The first gene encodes the nucleoprotein (N protein) which associates with the viral genomic and antigenomic RNAs to form the helical nucleocapsid. The paramyxoviral nucleocapsid assembly entirely covers the viral genome, protecting it from detection and degradation by host factors and serving as the template for viral mRNA transcription and genome replication. Here, we determined the cryoEM structure of the recombinantly expressed, full-length, and tag-free HeV N protein in complex with E. coli host-derived RNA. Following cryoEM data collection, a multimeric HeV N protein double-ring assembly was resolved to 3.5 Å resolution, enabling the building and refinement of an atomic HeV N protein model.

Subsequent 3D refinement of a curated particle stack comprising 5638 particles and using D14 symmetry resulted in a 3.5 Å resolution cryoEM density map, revealing a previously uncharacterised multimeric nucleoprotein assembly. In the HeV N protein assembly two rings stack ‘bottom-to-bottom’, where the globular N-terminal domains (NTDs) intercalate to form a dimer of tetradecamers. Each tetradecameric ring has a diameter of approximately 20 nm and is topped with the C-terminal arms (Ct-arms) which cover parts of the globular C terminal domains (CTDs). The double ring assembly is approximately 12.5 nm tall, and each ring has an aperture formed by the Ct-arms that is approximately 7 nm wide. The HeV N protein double-ring assembly is formed through extensive lateral interactions in each tetradecameric ring as well as intercalating interactions between two tetradecameric rings. A defining feature of this HeV N protein double-ring assembly is the gear-wheel interface between the two tetradecameric rings. This intercalation zone consists solely of residues in the NTDs of N protomers in the top ring and N protomers in the bottom ring (indicated by the lower-case n). The Ni protomer contacts two protomers in the bottom ring (ni and ni+1), with a total calculated buried surface area of ~ 545 Å2. A clear, reciprocal hydrogen-bonding interface exists between Ni and ni+1 with the residues Lys120, Glu123, and Glu124 where the two Glu residues in Ni form a tab that interacts with the Lys residue in ni+1 and vice versa. The dimer of tetradecameric rings that form the HeV N protein double-ring assembly is, to our best knowledge, a unique paramyxoviral N protein architecture lacking formal description in the current literature.

>MSDIFDEAASFRSYQSKLGRDGRASAATATLTTKIRIFVPATNSPELRWELTLFALDVIRSPSAAESMKIGAAFTLISMYSERPGALIRSLLNDPDIEAVIIDVGSMLNGIPVMERRGDKAQEEMEGLMRILKTARESSKGKTPFVDSRAYGLRITDMSTLVSAVITIEAQIWILIAKAVTAPDTAEESETRRWAKYVQQKRVNPFFALTQQWLTEMRNLLSQSLSVRKFMVEILMEVKKGGSAKGRAVEIISDIGNYVEETGMAGFFATIRFGLETRYPALALNEFQSDLNTIKGLMLLYREIGPRAPYMVLLEESIQTKFAPGGYPLLWSFAMGVATTIDRSMGALNINRGYLEPMYFRLGQKSARHHAGGIDQNMANKLGLNSDQVAELAAAVQETSVGRQDNNMQAREAKFAAGGVLVGGGEQDIDEEEEPIEHSGRQSVTFKREMSMSSLADSVPSSSVSTSGGTRLTNSLLNLRSRLAAKAIKESTAQSSSERNPPNNRPQADSGRKDDQEPKPAQNDLDFVRADV[28x]> MADVAGTSNRDFRGYILSVQAEEQYNYNNSLNGEVSVWVYAYYSDGSVLVINKNSQYKVGISETFKALKEYRE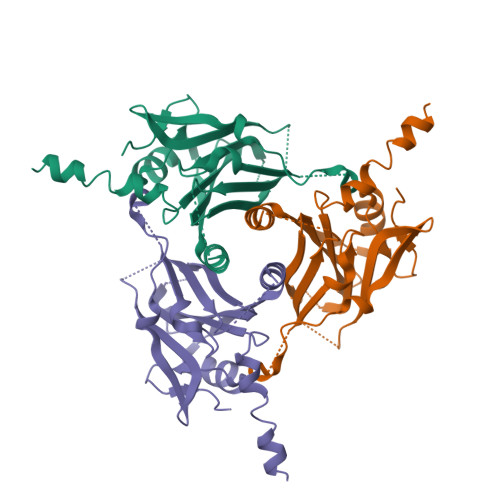GQHNDSYDEYEVNQSIYYPNGGDARKFHSNAKPRAIQIIFSPSVNVRTIKMAKGNAVSVPDEYLQRSHPWEATGIKYRKIKRDGEIVGYSHYFELPHEYNSISLAVSGVHKNPSSYNVGSAHNVMDVFQSCDLALRFCNRYWAELELVNHYISPNAYPYLDINNHSYGVALSNRQ> GSGQDIQL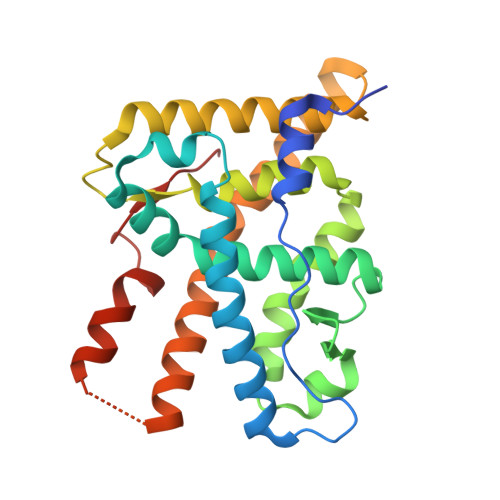IPPLINLLMSIEPDVIYAGHDNTKPDTSSSLLTSLNQLGERQLLSVVKWSKSLPGFRNLHIDDQITLIQYSWMSLMVFGLGWRSYKHVSGQMLYFAPDLILNEQRMKESSFYSLCLTMWQIPQEFVKLQVSQEEFLCMKVLLLLNTIPLEGLRSQTQFEEMRSSYIRELIKAIGLRQKGVVSSSQRFYQLTKLLDNLHDLVKQLHLYCLNTFIQSRALSVEFPEMMSEVIAAQLPKILAGMVKPLLFHKK The small 3-O-sulfated galactose head group of sulfatides, an abundant glycosphingolipid class, poses the (sphinx-like) riddle on involvement of glycan bridging by tissue lectins (sugar code). As an attractive possibility, the concept of the sugar code considers the glycan part of glycosphingolipids as a biochemical message anchored in the membrane, and thereby presented on its surface ready for being ‘read’ by receptors (Gabius and Roth, 2017; Kaltner et al., 2019). Like the glycosphingolipids, known endogenous receptors for their glycan part (lectins) present their own mysteries (Ledeen et al., 2018). Especially the occurrence of diverse types of modular architecture is not yet fully understood in functional terms. As illustrated in the bottom part of Figure 1 for vertebrate galectins, three distinct forms are found (García Caballero et al., 2020; Kaltner et al., 2017).

Respective testing disclosed aggregation also for Gal-8 (bottom, left). The two tandem-repeat-type galectins thus appear to use a compensatory contact for acquiring stability, and here sphingosine's hydroxyl group comes into play as a possibility. A means to test the validity of this hypothesis is crystallographic study, if a complex of a galectin CRD with synthetic sulfatide-1 could be obtained. Clear electron density for the head group structure was obtained, whereas the amide's acyl chain appeared rather mobile, so that a profiling of the head group's contacts became possible. As depicted in Figure 4A on two levels of magnification, the galactose moiety with its sulfate was central to contact building. In this position, sphingosine's hydroxyl group and side chains of Arg69/Glu89, together with a water molecule, are connected by hydrogen bonding. It hereby appears to functionally substitute the 3′-hydroxyl group of the glucose part of lactose. The data obtained by crystallography with the synthetic head group are first evidence that a non-glycan determinant, here sphingosine's hydroxyl group, is involved in sulfatide pairing with a galectin via water-mediated contacts, as the 3-OH group of glucose of the canonical ligand lactose otherwise does by direct hydrogen bonding. Structurally, sulfatide recognition by galectin-8 is shown to involve sphingosine's OH group as substitute for the 3′-hydroxyl of glucose of lactose.

> LNNLQNIIYNPVIPFVGTIPDQLDPGTLIVIRGHVPSDADRFQVDLQNGSSMKPRADVAFHFNPRFKRAGCIVCNTLINEKWGREEITYDTPFKREKSFEIVIMVLKDKFQVAVNGKHTLLYGHRIGPEKIDTLGIYGKVNIHSIGFSFSSDLQST>GSHMPGPVARLAPQAVLTPPSAASLFLVLVAGDSDDDRATVCDVISGIDGPLKAVGFRELAGSLSCVVGVGAQFWDRVSASSKPAHLHPFVPLSGPVHSAPSTPGDLLFHIKAARKDLCFELGRQIVSALGSAATVVDEVHGFRYFDSRDLLGFVAGTENPTDDDAADSALIGDEDPDFRGGSYVIVQKYLHDMSAWNTLSTEEQERVIGRTKLENVELDDDAQPSNSHVTLNTIVDDDGVEHDILRDNMAFGSLGEAEYGTYFIGYAKDPAVTELMLRRMFLGEPPGNYDRVLDFSTAATGTLFFVPSRDVLESLGDE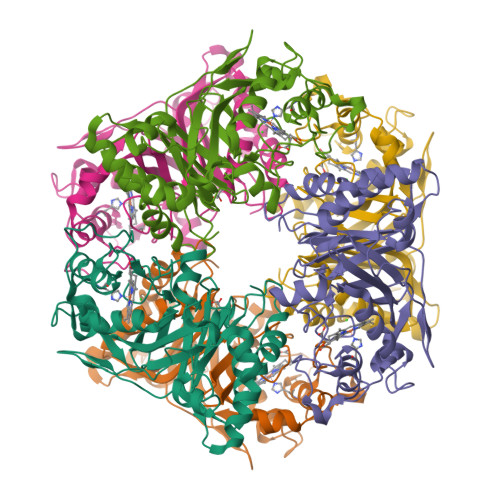PAGAESAPEDPVEPAAAGPYDLSLKIGGLKGVSQ[3x]N-{[4-(2-amino-1H-imidazol-4-yl)phenyl]methyl}-2-[4-(benzenesulfonamido)phenyl]acetamide | C24 H23 N5 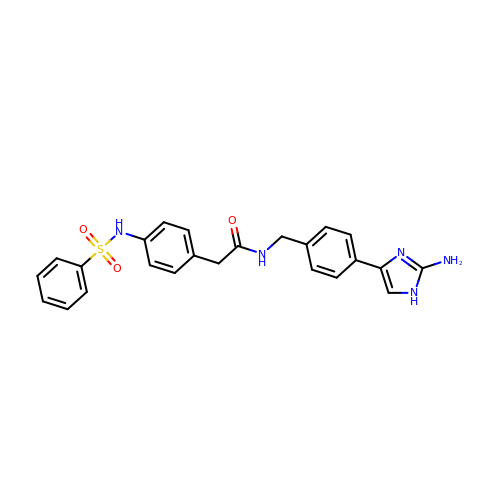O3 S | SVDHOWDKPFNTMO-UHFFFAOYSA-N> IDDEMFYDDHLE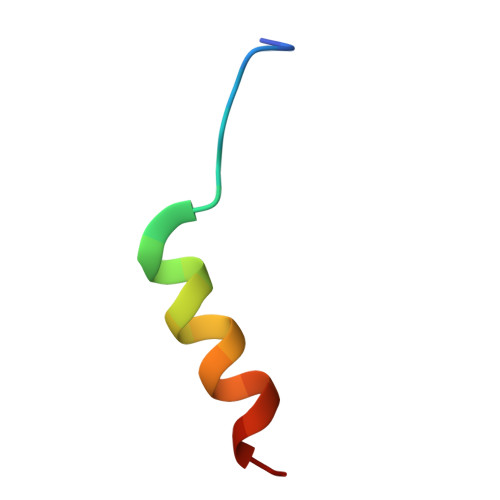AYFEQLAIPG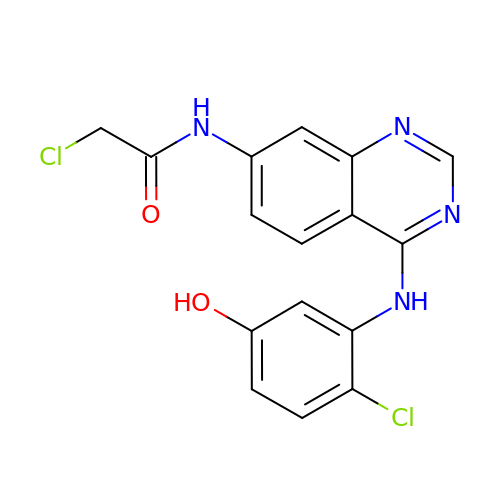2-chloranyl-~{N}-[4-[(2-chloranyl-5-oxidanyl-phenyl)amino]quinazolin-7-yl]ethanamide | C16 H12 Cl2 N4 O2 | GVQPPCNXPVHIRJ-UHFFFAOYSA-N> KYSKRIAWMKTTICDSLQLKDMIVEESFQYEKNKNLLEQFLSGEGLNKIFAYYQVQEQAQNDDIKDTGAQDPVLFFTTGDLEKIQDKAVWFLRITNPADDKKKASQQDGNDNDIIFGEITPNTVPMLNALMESVYSRQIDHIITEKIQFWGVAEEEQVLEFQQHSNKFSSEVREAINLMSPGTEHFKLDYEAISGLSESEKMQHYEMKFNEWINLISSQLNDDSEVRKDEKDAGPATELIYWRSRMQKITNWSEQLKSKDFQIVKASLQRHKNHDNQRPRGDESLSKLMMEYNRLDLLLTDKLNEAKDNVKYLTTLEKFIEPLYNGTPQQIIDTLPALMNAIKMIHTIARFYNTTDKMTGLFIKITNQMIKNCKDRILNKKDNGDNPSLYKMIWEQDPAELIEVLGSCIKLYCEYKKCYNDTKEKVADMPKGKTFDFSDAQIFGKFDTFVRRLQKLIEIFSNIQQFNALAKHNLEGMDVLTNKFKKIIDDFKKKGHNLLDTANNKFDRDWVEFNVEISHLDGELQNFIDNNFNRFRNIEYSLKLLHKFQSTIKRDSLKHNLTSRYNAILHNYATELDTIQRVFQDQKSNPPLVRNMPPEAGKIIWARHLFQKITGPINIFPENVINSTEIRRYYGSYNTLGKQLTIYEMWFYQDWVNKIEQSKAALQATLIVRHDENKKLYVNFDLEIMQLIREAKCLDRQGIEIPESARIILLQEDKFKTYYNELLYALKEYERINSKIKPICKNLLLPHIEDLDLKLRPGMVTLTWTSMNIESYLYYVHQGLKKLEQLIINVNDIIENRIENNLKTVSKVVLVHLPQDTKPLSLDSFVQLQEEYINSKTDFLTSKNVEVERAVDDLLQTIMLYPLDPHVDPVLPEETKRIKRYYFWYFYQALLNSTQNSLNAMKYRVCGKKIPGANTLQNLKPFFQVEVQLNGDKVTLNPSLQEIQKSINRAATAVLRCSKHLYNWDQQNKDSTDKATFYDMIACDKEIVKVILLLTGSIQGTKNKVNEFLSGFTKFEWLCKESIQESIKKFSKNGPTLQNYEDQLKKFSQIEEEIEKIVPTYKIGAMELMTHNICTSLSTWAKEWKLQYSQDLHKRARQLLDSLTEQTKMLSTKLSKPVKDIDSLGYVMETLEQIRKEQAEIDMKFNPVQEMYSLLDNYLPGGITDKDEMDARSLLRRNWDILIQQAEIKGKEYQHKQAIYLKELKQSIKDFTNQVSIFRRDYEKNGPMVEGISPAEAMERLRRFEDEYDVKYQMYKINARGENLFGLQNQKYPELEKTDAEIKNLNKLYNLYDSVIKNIQQFKEKSWQDVSKDDLAKMEEDAGKYGEQCSRLPKDLKEWQAYRDLKNYIDSLREQLPLIISLKKPSIMPRHWEKIKEITNTKLNYENPDQFYIEEIMGAKLLDFREDIEDITESADKQLKIRTGLDEINLYWNDMQFQFGIWGKRDVPCMLNGLIVGTILERLEEDQLQLSTFNS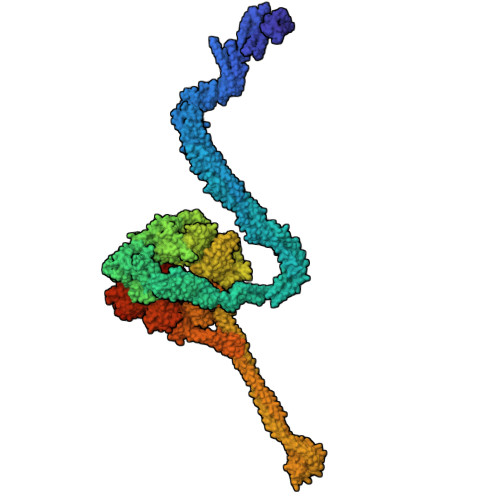QRHVTPFKAEVENLIRTFSDVNDTLDMWVKVQKLWTSLEPVFTGGDIARQMPLQAKQFQGIDKNWMKIMEKAVETKKVIPCCQNDMLKDFLPDLNRKLEDCQKMLEAYLEGKRKKFPRFYFVSNPTLLKILSQGSEPTSIQEDFEKLFDAITKVTFESAKDKKNPALKQITQIQQVIGRNEENISLTGYYVKCEGNIEDWLKKLEQNMQQTLKDIASAAAQQVFQVGLKEFVSSQASQIALLGLQILWTSKVNEGLERLSRNERNAMDIKRNEIKEHMNILSSMCLEDLNGAVERTKVETLVTIQVHQKDISMDLKCKDVNDFEWQKQTRIAWKTDIDECIISITDWDSPYSYEFLGAKERLCITPLTDRCYITLAQAMSMYYGGAPAGPAGTGKTETVKDLGRTLGVFVVVTNCSDQHRYRDMAKIFKGLVQSGLWGCFDEFNRIDLEVLSVVAMQVESITTARKQHMKKFMFPEEEIEIELIPTVSYFITMNPGYAGRQELPENLKVLFRGVSMMVPDREIIIKVKLASVGYLQIDLLAKKFNVLYRLCEEQLSKQRHYDFGLRNILSVLRTAGNTKRQEIKSDEEMLLMRSLRDMNLSKLVADDIPLFNGLLADIFPKLKEVPKKLYPDVEKKIPEEINAESYLINTPSFQLKIIQLYETCLVRHGFMLVGPTGSGKSTIMKILTEVLTKLGSPHKIVIMNPKAITAEQMYGVKSEISDDWIPGVFSTIWAKSNNRALKHTTWITCDGPVDAIWIENLNTVLDDNKILTLANGERIAMTENCKVVFEVENLNNASPATVSRCGQVYVSPTDLGYEAVIEGWIRNRKASGRAEESDKLGNILRKYLINMRFIELQSKECKEPMMDTSPVISVINILNLLTGCLQYFVQTQRTLSEQEYEKFIVYSMAWAIGGIYEAQDRVRFHELLLAKNAPIPQKGKENETVFDYYVSQDYLDWKICSPEEWVPPQSLQFSQLLLPTLDSFRAEMLLNFILTQPKSHTCSNSALLIGGSGTAKTSSVLLYCNKFDPQKMLFKRTNFSSATSPFMFQSTIEAECDFKVGKEFAPPGNKMMTIFIDDMSMPFVNKWGDQITLELVRQLIETGGFYMLDKTQRGNQRKMKNLQYIGAMNHPGGGRNDIPNRLKRQFFIFNMILPLSIEGIYGPIIKHMFKQKYFSDSTYKVIESLTSATIALWNKVKSTMLPTPAKFHYVFNMRELSRIFKGILTCKKDTINDAPKSMKIKPELFLVGLWRHEAERVLADKLVNNKDKDTVMGYIQEVSLESFSQIENEILEKYSSEKTFLFCDFLRPDVINEDGIIEEEAPKIYEAIDSLTELRKRCNFLLSFYNDRNPSKKMPLVLFDDALKHLLRISRIIRQPRSSGLLVGVGGSGKQSLTRLAGFIGKNLIQQIIVTKTYSDKDLKEDIKKGFDDAGHLGKQVTFLMTDSEVKKEEFLEYINMVLSTGEIPNLLAKDEREVWLGDISQAYCKEKNLGNIDPPQSELWTYFVDRVRDNFHIMLCFSPVGQKFRERARKFPALFNECTIDWFLPWPEEALVSVAETFIKNFDKLDTKEETKQELMKHMGNVHLMVNEICDEYYQKMRRQVYVTPKSFLSYLNSYKTLYIEKYDELDQQEESFKIGLNKIQEATITINQMEISLKEEEIQLNEATEKTNQLLANLDKESKKANQKGEEVAATNKQCEIQAEQISKEKEEAERELEAALPALRRAQEAVDSIESKDIVELKANKKPLDIIKYIMDAVLVFFKARLIPIQIEERVFNKKEGKAVLFLKESYDESGIQTLGDMNFMKKLKEFEKDSINEETIELLEPYLNQSEDWFNDTFATKASKAAAGILKWAFAIYEYHQKSKIVKPKRIQVAIAEGRQAIALKELEKAREDLAQIQAYIKNLKDVYTKQMEEKNELEMKAAKTKKKINTARTLITSLSGEKDRWGKGAQDISDQKRKLVGNVSLSTAFISYCGPFNAEYRNKLAQQRFVVDMKKRGVPVTPGLELTSFLIDDATIGEWNLQGLPKDDLSIQNGIMVTNSARYPLFIDPQGQGQNWIRNKLSASIIPERCITTLSHPKFKDMFLKYCMESGLTLIVENIENEVDPMMDPVLERQIIVKGKTQFVNVAGTEMELSKEFKLFMTCRLANPSFSPELSAKTTIIDFTVTQSGLEQQLLGKVISKEQKALEDSLNQLLADVNQNQKDLQRLDKNLLERLINSQGNLLDDTELMDVLNNTKTQAKEVAAKLIDAEIKTKEINEKREQYRPVAIRGSAIYFTMIEVSLVNWMYNSSLEQFLKLFIESIDLSEKAQLPSNRVKNIISFLTFHVYRYVNRGLFEKDKITFILMMAFKILTTAGTISSGDVSLFLKSGDALDIKSERQKQISYLEDNQWLNILALSKHTFSGQTLPFFKELPDLISRSENQWRNWIDKNDPENFPIPDFAESINQEKEIGSFISLCLVRSLRNDRTLIATQNFISNVLGKEFTDPISYPIEGIWQESSNMDPVLFLLSAGADPTSSIDELAKKKKKFPCEKVSMGEGQERVARQVIMKGFVEGGWVILQNCHLGLKFMEEIETLVSPINQIHEDFRLWITCEQHPKFPLGLLQKTLKVTNEPPKGLKAGLYKTFTTIITQEFIDKVDHSNWRSLIFTICFLHSIVIERKKFGPLGWCVPYEYNYSDLEASLLYIEKYLTNLMSTPQPNSHNLPISMNVVRYMICEVQYGGRITDDLDRELFITYGETYLKDGIFGNDYFFYDIMVDGSGQKFKYRIPQNPSAELIKYQEYIAKVPTVDNPEVFGLHSNADLTFRLKESKEMINTVMETRPKDSSVGGGKTREEIVQDKAKDMLKNLPPDYNDVEVRELVSKLGGPNPKTSTERGMTVPLNIFLYQEVTRMQRVIGLVRKTLQDTILAIDGQIIMTPEILEAINAIYDAKVPNSWLYDPSGAEISWLLPNLGSWSTSLSDRNKQLNDWLRSGQRPILFWLTGFFNPQGFLTGMKQEVTRNHKKGDGKGGEAWSLDDVVYSTTVKEREKEKDIEQPPAEGVYIKGLYLEGCKWSKNGLDDSDPKKIFADLPILHVSAINKKKTNEQDRMSNTYLCPVYKYPKRTDKYLIFRVGLPCEGSNNPSHWKLRGVALLCST>[2x]MIICSVDIGIKNPAYAIFNYDNTSNTI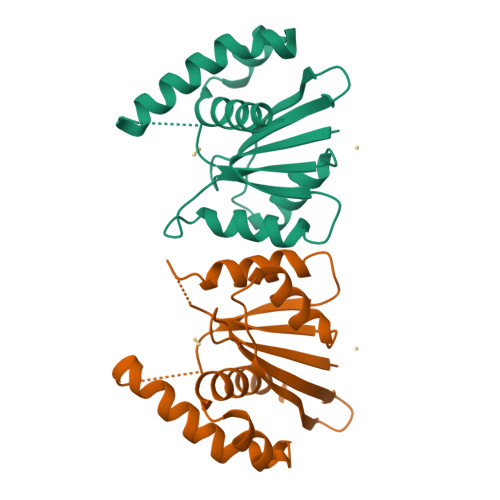KLIAIEKSDWTKNWERSVARDLTRYNPDVVILEKQGFASPNSKIIYFIKGFFYNSNTKVIVRNPTFKGGSYRNRAAASIDVFIQKISEYTDYKNDILNKYTKLDDIANSFNLGLSYMESLL>[4x]PPYTVVYFPVRGRCA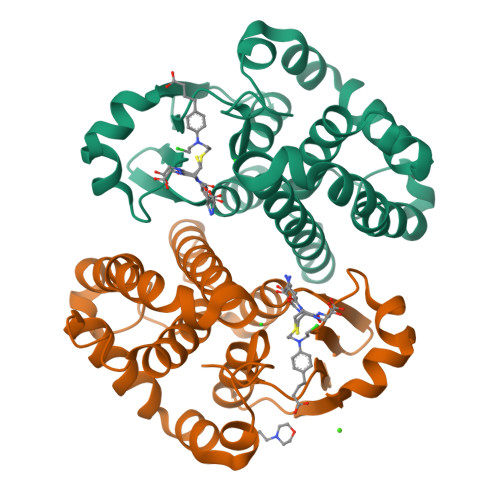ALRMLLADQGQSWKEEVVTVETWQEGSLKASCLYGQLPKFQDGDLTLYQSNTILRHLGRTLGLYGKDQQEAALVDMVNDGVEDLRCKYVSLIYTNYEVGKDDYVKALPGQLKPFETLLSQNQGGKTFIVGDQISFADYNLLDLLLIHEVLAPGCLDAFPLLSAYVGRLSARPKLKAFLASPEYVNLPINGNGKQ(7S,10aR)-1-methyl-4-{4-[(5R)-1,1,5-trihydroxy-4,4-dimethyl-1,6,10,15-tetraoxo-2-oxa-7,11,14-triaza-1lambda~5~-phosphahexadecan-16-yl]phenyl}-3,5,6,7,8,9,10,10a-octahydrocycloocta[d]pyridazin-7-yl [(5R)-1,1,5-trihydroxy-4,4-dimethyl-1,6,10-trioxo-2-oxa-7,11-diaza-1lambda~5~-phosphatridecan-13-yl]carbamate (non-preferred name) | C42 H68 N8 O17 P2 | 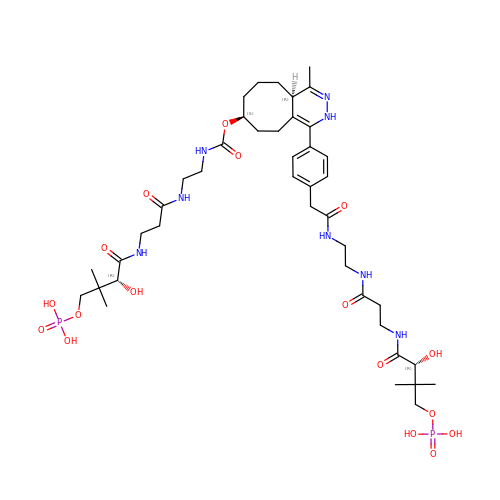NIBTULRMWBVSTM-MEITYLAXSA-N> SCPPTKFQCRTSGLCVPL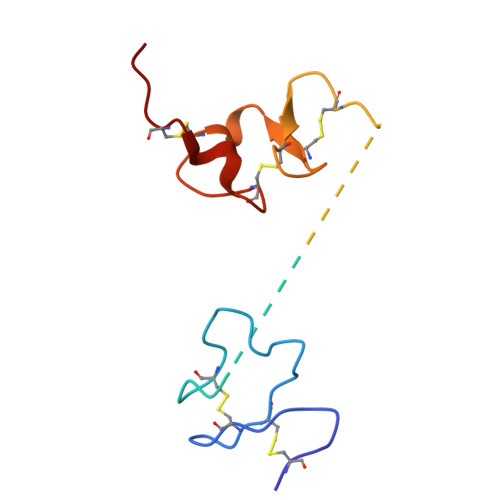TWRCDRDLDCSDGSDEECRIEPCTQKGQCPPPPGLPCPCTGVSDCSGGTDKKLRNCSRLACLAGELRCTLSDDCIPLTWRCDGHPDCPDSSDELGCGTNE> MFERFTDRARRVVVLAQEEARMLNHNYIGTEHILLGLIHEGEGVAAKSLESLGISLEGVRSQVEEIIGQGQQAPSGHIPFTPRAKKVLELSSREAPQLGHNYIGTEHILLGLIREGEGVAAQVLVKLGAELTRVRQQVIQLLSGYKLAAALEHHHHHH

ClpC1 is an ATP-dependent homohexamer that is responsible for substrate recognition and unfolding. ClpC1 is a 95 kDa caseinolytic AAA+ protein with an N-terminal domain (NTD) and two nucleotide-binding domains (D1 and D2). The essential ClpC1–ClpP1–ClpP2 proteasome complex of Mtb has recently become the focus of several drug-discovery campaigns. The NTD (amino acids 1–145) has been studied extensively to determine the most critical residues for the binding of ClpC1 to several natural cyclopeptides with potent anti-TB activity.

Since single mutations at sites Leu92 and Leu96 of ClpC1 caused a reduced binding affinity for ECU, the crystal structure of an engineered double mutant was solved to investigate the mechanism of resistance. Since the L92S mutation had a lower affinity for ClpC1-NTD, it was chosen for the double mutant. Superposition of the structures of ClpC1-NTD-L92S/L96P and the ECU complex resulted in an overall r.m.s.d. of 1.12 Å or of 0.71 Å without the three N-terminal residues. The N-terminus of ClpC1-NTD-L92S/L96P is a curved loop in approximately the same orientation as in the RUF-I complex and apo forms. Looking into the changes at the mutation sites, a distortion (‘kink’) in the helical backbone induced by proline and the missing nitrogen bond acceptor of the carboxyl of Ser92 was observed. This C=O bond protrudes out of the helix axis and is at an approximate hydrogen-bonding distance from NH2 of Arg4. Accordingly, the L96P mutation apparently does not have a significant effect on the length of helix 6 as both the ClpC1-NTD-L92S/L96P and ECU complex structures terminate this helix at residue 97, while some other structures terminate at position 98. This subtle alteration is significant in relation to the binding of ECU, as the conformation of Arg4 may be important for the three previous residues of the N-terminus (Met1-Phe2-Glu3) to adopt the extended ‘ECU-binding’ conformation for site 1. However, in ClpC1 the L96P mutant confers ECU resistance, as do the L92S and L92F mutations. As shown in Fig. 3(b), it was observed that the double mutation L92S/L96P introduced a kink in helix 6 and replaces a hydrophobic residue (Leu) with a more polar Ser.>[2x]MGKAVIAIHGGAGAISRAQMSLQQELRYIEALSAIVETGQKMLEAGESALDVVTEAVRLLEECPLFNAGIGAVFTRDETHELDACVMDGNTLKAGAVAGVSHLRNPVLAARLVMEQSPHVMMIGEGAENFAFARGMERVSPEIFSTSLRYEQLLAARKEGATVLDHSGAPLDEKQKMG;>TVGAVALDLDGNLAA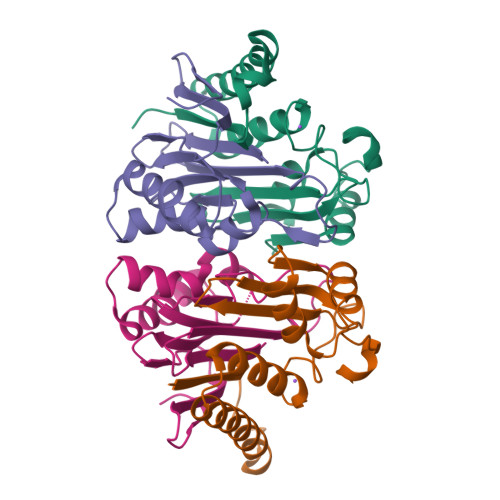ATSTGGMTNKLPHTVGPQPLVGAGCYANNASVAVSCTGTGEVFIRALAAYDIAALMDYGGLSLAEACERVVMEKLPALGGSGGLIAIDHEGNVALPFNTEGMYRAWGYAGDTPTTGIYREKGDTVATQ[2x]4-(4-chloro-2-{5-[(trimethyl-1H-pyrazol-4-yl)methyl]-1,3,4-oxadiazol-2-yl}phenoxy)piperidine | C20 H24 Cl N5 O2 | 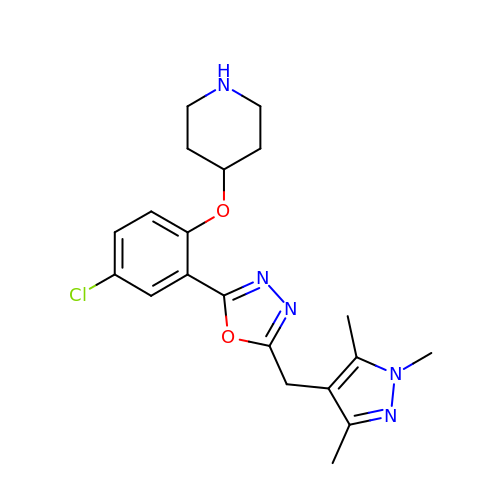AYWNZLSZEHOECC-UHFFFAOYSA-N>[2x]STQIGGMSLDQARTQLAPWTQRAAPIGADEYQQRIERARVLMRAQGVDALLIGAGTSLRYFSGVPWGASERLVALLLTTEGDPVLICPAFEEGSLDAVLQLPVRKRLWEEHEDPYALVVQAMDEQHAHALALDPGIAFAVHTGLRAHLGTAIRDAGAIIDG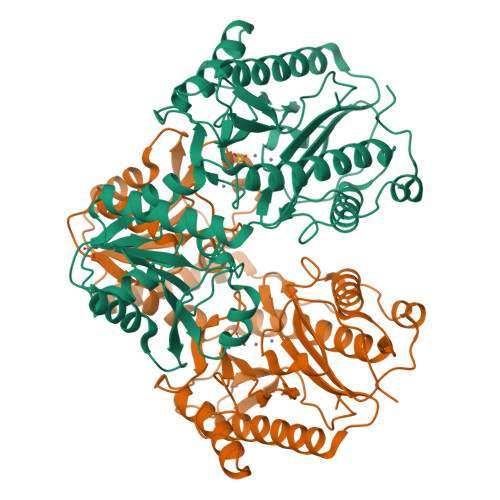CRMCKSPAELALMQQACDMTLLVQRLAAGIAHEGIGTDQLVRFIDEAHRALGADNGSTFCIVQFGHATAFPHGIPGVQHLRAGELVLIDTGCTVQGYHSDITRTWIYGTPSDAQQRIWELELAAQAAAFAAVRPGVACEAVDQAARAVLQAAGLGPDYRLPGLPHRTGHGCGLAIHEAPYLVRGNRQPLQPGMCASNEPMIVVPGAFGVALEDHFYVTDTGAQWFTPPSVAIDQPFA> FYR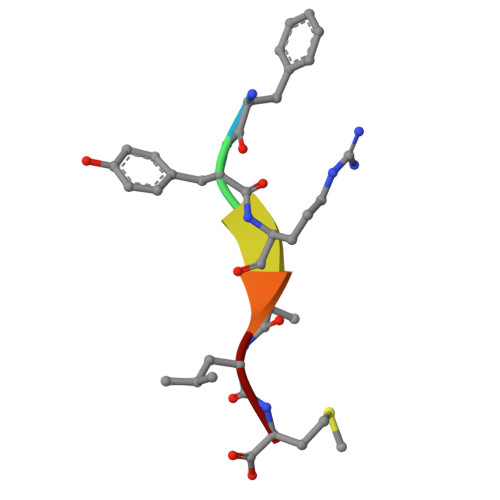ALM>MNTMLFSPYTIRGLTLKNRIVMSPMCMYSCDTKDGAVRTWHKIHYPARAVGQVGLIIVEATGVTPQGRISERDLGIWSDDHIAGLRELVGLVKEHGAAIGIALAHAGRKSQVPGEIIAPSAVPFDDSSPTPKEMTKADIEETVQAFQNGARRAKEAGFDVIEIHAAHGFLINEFLSPLSNRRQDEYGGSPENRYRFLGEVIDAVREVWDGPLFVAISASDYHPDGLTAKDYVPYAKRMKEQGVDLVDVSSGAIVPARMNVYPGYQVPFAELIRREADIPTGAVGLITSGWQAEEILQNGRADLVFLGAELLRNPYWPYAAA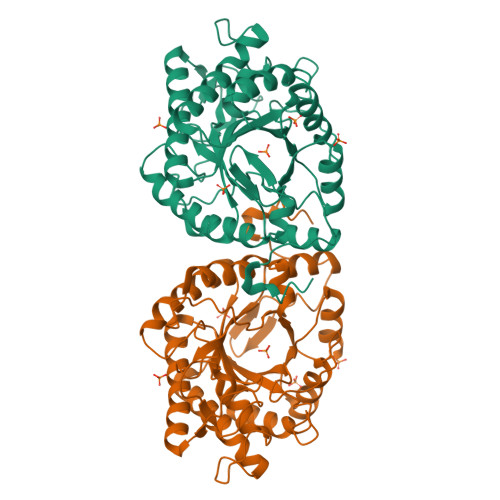RELGAKISAPVQYERGWRF[2x]>SMKLTIPELSLVVLIGSSGSGKSTFAKKHFKPTEVISSDFCRGLVSDDENDQTVTGAAFDVLHYIVSKRLQLGKLTVVDATNVQESARKPLIEIAKDYHCFPVAVVFNLPEKVCQERNKNRTDRQVEEYVIRKHTQQLKKSIKGLQREGFRYVYILNSPEEVEEV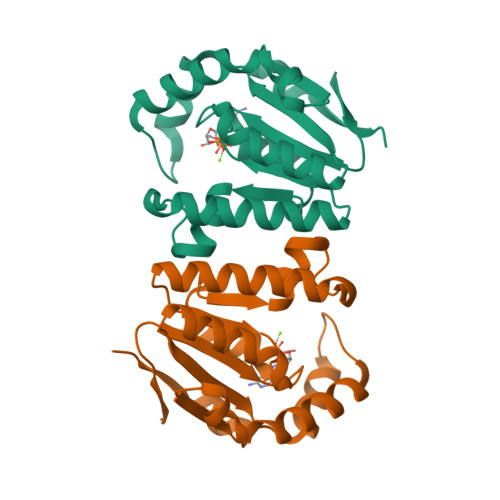VFERQP[2x]> MEDHGIVETLNFLSSTKIKERNNALDELTTILKEDPERIPTKALSTTAEALVELLASEHTKYCDLLRNLTVSTTNKLSLSENRLSTISYVLRLFVEKSCERFKVKTLKLLLAVVPELMVKDGSKSLLDAVSVHLSFALDALIKSDPFKLKFMIHQWISLVDKICEYFQSQMKLSMVDKTLTNFISILLNLLALDTVGIFQVTRTITWTVIDFLRLSKKENGNTRLIMSLINQLILKCHCFSVIDTLMLIKEAWSYNLTIGCTSNELVQDQLSLFDVMSSELMNHKLPYMIGQENYVEELRSESLVSLYREYILLRLSNYKPQLFTVNHVEFSYIRGSRDKNSWFALPDFRLRDRGGRSVWLKILGITKSLLTYFALNRKNENYSLLFKRRKCDSDIPSILRISDDMDTFLIHLLEENSSHEFEVLGLQLCSFYGTLQDFTKSFAEQLKELLFSKFEKIQCFNWVCFSFIPLLSQKECELSNGDMARLFKVCLPLVKSNESCQLSCLLLANSIKFSKQLLSDEKTINQIYDLYELSDILGPILVTNESFMLWGYLQYVGKDFQSMNGISSADRIFEWLKSKWNQLRGTDAKQDQFCNFISWLGNKYDPENPFNDKKGEGANPVSLCWDESHKIWQHFQEQREFLLGVKPEEKSECFNTPFFNLPKVSLDLTRYNEILYRLLENIESDAFSSPLQKFTWVAKLIQIVDNLCGDSTFSEFIAAYKRTTLITIPQLSFDSQNSYQSFFEEVLSIRTINVDHLVLDKINMKEIVNDFIRMQKNKSQTGTSAINYFEASSEDTTQNNSPYTIGGRFQKPLHSTIDKAVRAYLWSSRNKSISERLVAILEFSDCVSTDVFISYLGTVCQWLKQAIGEKSSYNKILEEFTEVLGEKLLCNHYSSSNQAMLLLTSYIEAIRPQWLSYPEQPLNSDCNDILDWIISRFEDNSFTGVAPTVNLSMLLLSLLQNHDLSHGSIRGGKQRVFATFIKCLQKLDSSNIINIMNSISSYMAQVSYKNQSIIFYEIKSLFGPPQQSIEKSAFYSLAMSMLSLVSYPSLVFSLEDMMTYSGFNHTRAFIQQALNKITVAFRYQNLTELFEYCKFDLIMYWFNRTKVPTSKLEKEWDISLFGFADIHEFLGRYFVEISAIYFSQGFNQKWILDMLHAITGNGDAYLVDNSYYLCIPLAFISGGVNELIFDILPQISGKTTVKYHKKYRLLMLKWIIRFTDLGSLTELRSTVEKLFPTSYLSPYLFENSSVSMRYQYPLHIPLALGATLVQTQFAHEKNNTHEFKLLFLSVITDLEKTSTYIGKLRCARELKYLFVLYENVLVKSSTLNFIIIRLSKFLIDTQIHDEVITIFSSLLNLADKNTFEIEPSLPNLFCKIFIYLRENKQLSPSFQQAIKLLEHRDLIKIKTWKYCLDAIFGNIVQDDIYENTELLDASDCGVDDVVLVSLLFSYARRPVASKIGCSLSKAAAINILKHHVPKEYLSKNFKLWFAALSRRILQQEVQRERSTNFNNEVHLKNFEMVFRHPEQPHMIYQRISTFNKEAELYDSTEVFFISECILTYLVGYSIGNSESEFCFRDNIMNENKDKVAPLDKDVLNAIYPLANNFGMESFICDTYLSVNEPYNCWLSKFARSLIHQISFNIPPIVCLYPLCKGSTAFCELVLTDLFFLSTTYDPKSCLNWSNRIFTQIAMLLHVKDSEIKLKMLFNVIKMIRMGSRCKERNCLRIYSSLDLQEICQISLKIKEFKFGYLLFEEMNMPNIREMNINTLQKIYECINDGDFLAGLPVPHSIEGVLNSINRIDSDTWKRFLFNNADFDANYTTSLEEEKESLIKATEDSGFYGLTSLLESRLSGSSDVYKWNLELGDWKLLTPKVVDSKAKGLYYAIKNLPQDVGFAEKSLEKSLLTIFDSRQHFISQTEWMDTLNAIIEFIKIAAIPQDVTSFPQTLMSIMKADKERLNTIDFYDHKTTLKSRHTLMNVLSRNSLDENVKCSKYLRLGSIIQLANYVQLAIANGAPQDALRNATLMSKTVKNIAKLYDDPSVVSQIEKLASFTSANALWESREYKAPVMIMRDLLAQNEKNISESILYDDFKLLINVPMDQIKARLVKWSSESRLEPAAAIYEKIIVNWDINVEDHESCSDVFYTLGSFLDEQAQKLRSNGEIEDREHRSYTGKSTLKALELIYKNTKLPENERKDAKRHYNRVLLQYNRDSEVLK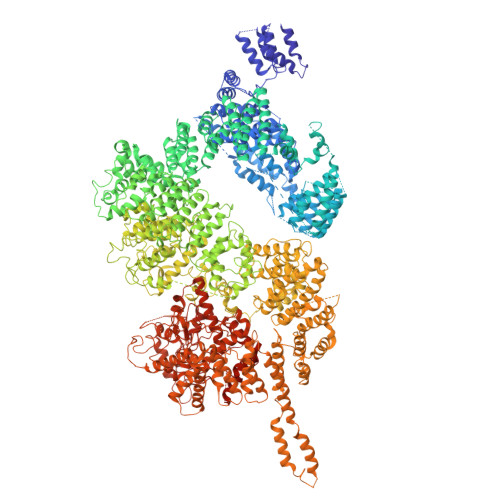ALLLQKEKFLWHALHFYLNTLVFSNRYDNDIIDKFCGLWFENDDNSKINQLLYKEIGTIPSWKFLPWVNQIASKISMEENEFQKPLQLTMKRLLYKLPYDSLYSVMSILLYEKQSNKDTNISQKIQAVKKILLELQGYDRGAFAKKYLLPVQEFCEMSVELANLKFVQNTKTLRLANLKIGQYWLKQLNMEKLPLPTSNFTVKSSADGRKARPYIVSVNETVGITTTGLSLPKIVTFNISDGTTQKALMKGSNDDLRQDAIMEQVFQQVNKVLQNDKVLRNLDLGIRTYKVVPLGPKAGIIEFVANSTSLHQILSKLHTNDKITFDQARKGMKAVQTKSNEERLKAYLKITNEIKPQLRNFFFDSFPDPLDWFEAKKTYTKGVAASSIVGYILGLGDRHLNNILLDCSTGEPIHIDLGIAFDQGKLLPIPELVPFRLTRDIVDGFGVTGVDGLFRRSCERVYAVLRKDYVKVMCVLNILKWDPLYSWVMSPVKKYEHLFEEEHEITNFDNVSKFISNNDRNENQESYRALKGVEEKLMGNGLSVESSVQDLIQQATDPSNLSVIYMGWSPFY>GSMGNYMGNPWTEYMAKYDIEEVHGSGIRVDLGEDAEVAGTQYRLPSGKCPVFGKGIIIENSKTTFLTPVATGNQYLKDGGFAFPPTEPLMSPMTLDDMRLLYKDNEDVKNLDELTLCSRHAGNMIPDNDKNSNYKYPAVYDDKDKKCHILYIAAQENNGPRYCNKDESKRNSMFCFRPAKDISFQNLVYLSKNVVHNWEKVCPRKNLQNAKFGLWVDGNCEDIPHVNEFSANDLFECNKLVFELSASDQPKQYEQHLTQQAKDIGAGPVASCFTTRMSPPQQICLNSVVNTA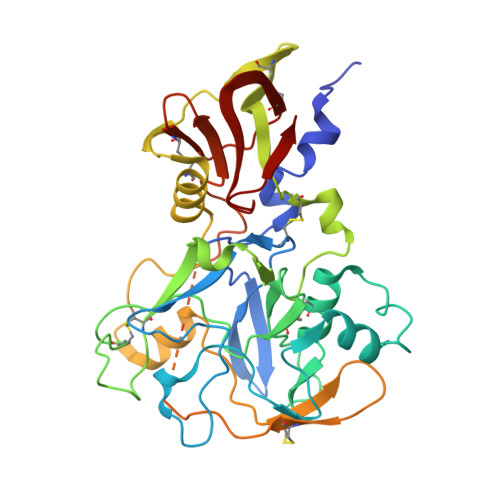LSGGSGGGNAAMIKSAFLPTGAFKADRYKSHGKGYNWGNYNTETQKCEIFNVKPTCLINDKNYIATTALSHPIEVEAAA[2x]> MDKKNILPQQGQPVIRLTAGQLSSQ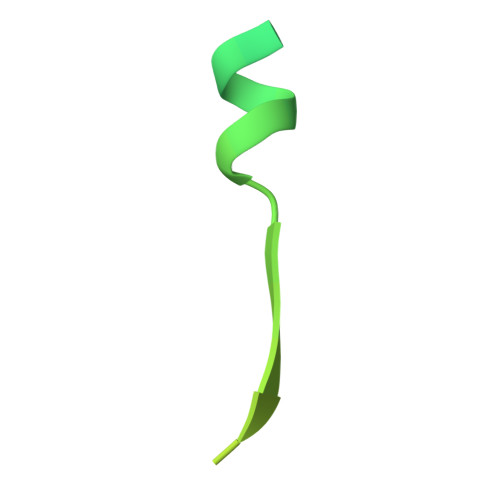LAELSEEALGDAGLEASKITACITFCAYDGELEHHHHHH> GPGSEFRERYELSEKMLSACNLLKYNIKDPKALASKDMRICLNTLQHDWFRVSSQKSAVPAMVGDYIAAFEAVSPDVLRYIINMADGNGNTALHYSVSHSNFQIVKLLLDADVCNVDHQ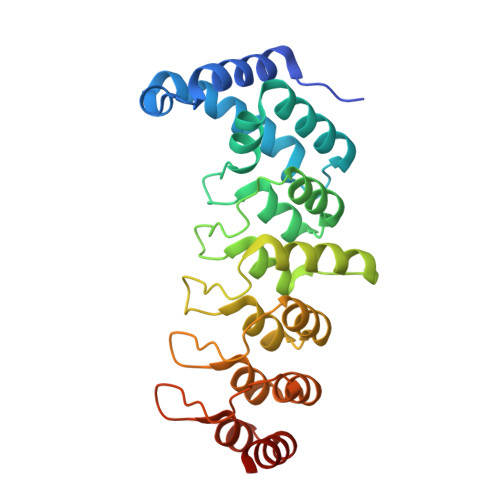NKAGYTPIMLAALAAVEAEKDMQVVEELFSCGDVNAKASQAGQTALMLAVSHGRIDMVKGLLACGADVNIQDDEGSTALMCASEHGHVEIVKLLLAQPGCNGHLEDNDGSTALSIALEAGHKDIAVLLYAHLNFSKAQ>MIEIIRSKEFSLKP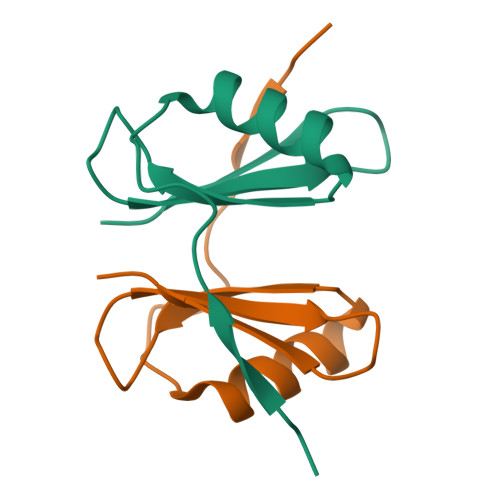MDSEEAVLQMNLLGHDFFVFTDRETDGTSIVYRRKDGKYGLIQTSEQHHHHHH[2x]>MMAGPLSGLRVVELAGIGPGPHAAMILGDLGADVVRIDRPSSVDGISRDAMLRNRRIVTADLKSDQGLELALKLIAKADVLIEGYRPGVTERLGLGPEECAKVNDRLIYARMTGWGQTGPRSQQAGHDINYISLNGILHAIGRGDERPVPPLNLVGAFGGGSMFLLVGILAALWERQSSGKGQVVDAAMVDGSSVLIQMMWAMRATGMWTDTRGANMLDGGAPYYDTYECADGRYVAVGAIEPQFYAAMLAGLGLDAAELPPQNDRARWPELRALLTEAFASHDRDHWGAVFANSDACVTPVLAFGEVHNEPHIIERNTFYEANGGWQPMPAPRFSRTASSQPRP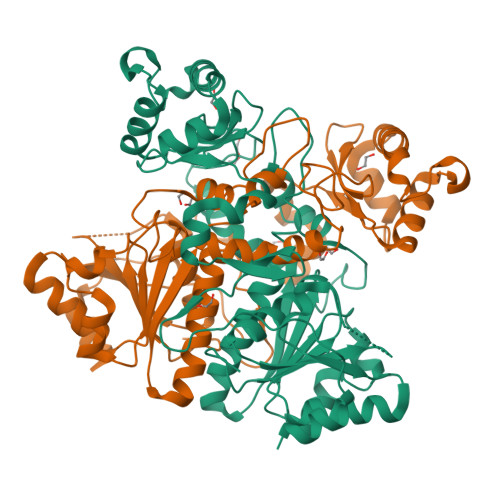PAATIDIEAVLTDWDGGSGC[2x]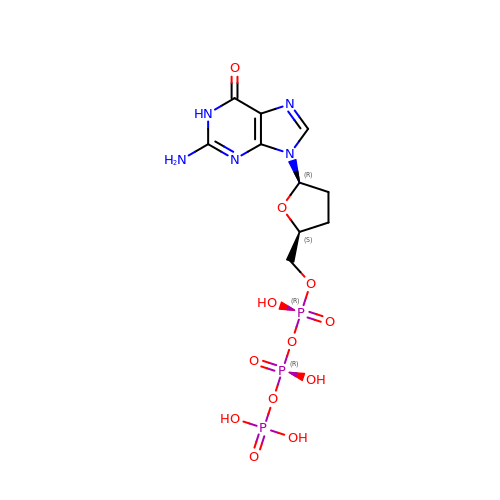2'-3'-DIDEOXYGUANOSINE-5'-TRIPHOSPHATE | C10 H16 N5 O12 P3 | HDRRAMINWIWTNU-NTSWFWBYSA-N> MDKINPDWAKDIPCRNITIYGYCKKEKEGCPFKHSDNTTATTINDVPPPIDVGEATTPTMTSVPKFNAKVSASFTPMTVGSDSLTTVTNTTSAATNATGNIAMAATSATASTVNPMINPIVNSSLVNNNNNNSNISISIPTTASSSNYDPFNAPIFTPSSTSSIHTNANAHSFPFPSIANSGGININATDDNSNNMSMANNVPPPMQPPPIESSNLKYPRIYPPPHSLLQYHLYAPEQPSSLKSLLKPNERSADQLFIPNNIREDLTKKNLSILQVFPSSGKVIPSIVQDYFNLVPLNFNNNDFLNKTTLFKVFSNYDGKAYVLKRLPNIDKSMNPNKISKIYQIWSKINCTNLIKFRDIFQTTKFGDLSICLVFDYYPNSLSLYDYHFVNFPKFPITNNYLWIYLVQLTNVINSIHSQNLSIGNTLNWRKVLI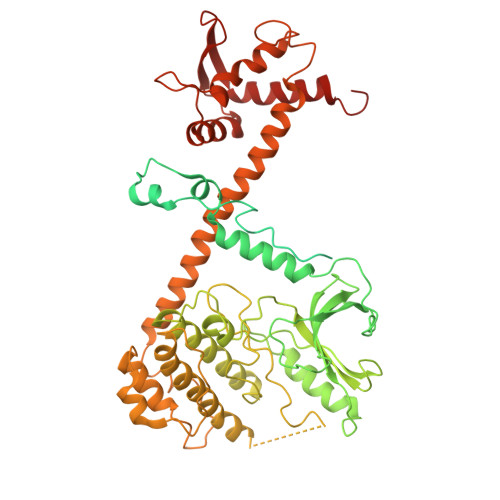TGDPGRIKLSHCNFMDLLFNDDTDTVVSSGGSTIEGQQQLDYKYLGELLFNLSINIENSNNNTAPKEYRLEEITPQSIDDMRQIDDKFKDVLKYLISDNGDSKKSIHDLTSHFYDKMFMVLESSQTYTEYMESVLSRELENGRLFRLVNKLNCIFGRIESRIDINWSESGTKFPIILFYDYVFHQVDSNGKPIMDLTHVLRCLNKLDAGIQEKLMLVTPDELNCIIISYKELKDLIESTFRSITQHHHHHHHHHH> LDPVFLAFAKLYIRDILDMKESRQVPGVFLYNGHPIKQVDVLGTVIGVRERDAFYSYGVDDSTGVINCICWKKL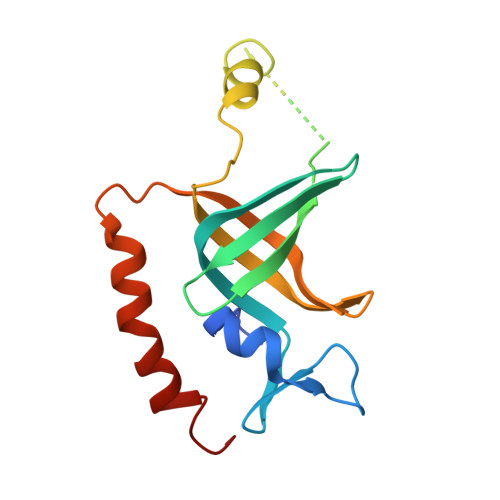NTESVSAAPSAARELSLTSQLKKLQETIEQKTKIEIGDTIRVRGSIRTYREEREIHATTYYKVDDPVWNIQIARMLELPTIYRKVYDQPFHS>[2x]CCGCCGCGCC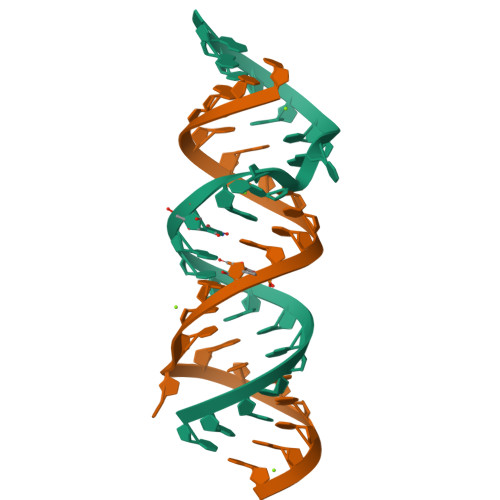AUGCCUGUGGCGG> SNASDKGKLSLQDVAELIRARACQRVVVMVGAGISTPSGIPDFRSPGSGLYSNLQQYDLPYPEAIFELPFFFHNPKPFFTLAKELYPGNYKPNVTHYFLRLLHDKGLLLRLYTQNIDGLERVSGIPASKLVEAHGTFASATCTVCQRPFPGEDIRADVMADRVPRCPVCTGVVKPDIVFFGEPLPQRFLLHVVDFPMADLLLILGTSLEVEPFASLTEA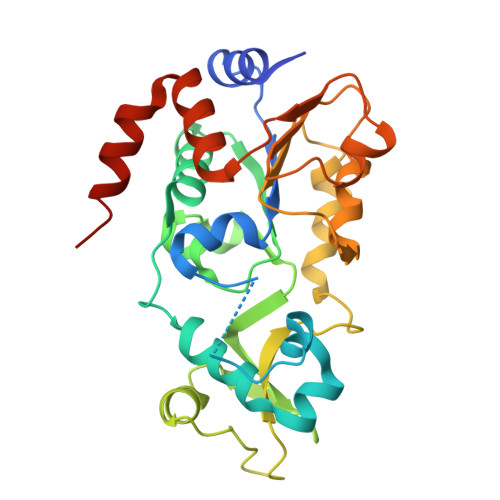VRSSVPRLLINRDLVGPLAWHPRSRDVAQLGDVVHGVESLVELLGWTEEMRDLVQRETGKLDGPDK> MSLNADFATEIEG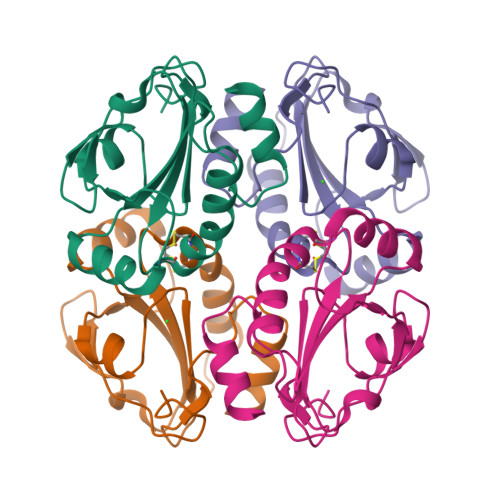KIVQASKLLPGQPAIDFEMLDVEGNVKHLADFKGKVIYIDLWATWCGPCIQESPAFEALGKKYVGKDIVFLPVSTDTTTKPWLRYLDGHKKELTQYHSNDVALKESWAIMYIPRFILIDKDFNIVNAYAPRPSSEEIGTLIDSVLNKEGHHHHHH> FFEEMTVYAPVPVPVNGNTHYTSESIERLPTGNGNISDLLRTNPAVRMDSTQSTSLNQGDIRPEKISIHGASPYQNAYLIDGISATNNLNPANESDASSATNISGMSQGYYLDVSLLDNVTLYDSFVPVEFGRFNGGVIDAKIKRFNADDSKVKLGYRTTRSDWLTSHIDENNKSAFNQGSSGSTYYSPDFKKNFYTLSFNQELADNFGVTAGLSRRQSDITRADYVSNDGIVAGRAQYKNVIDTALSKFTWFASDRFTHDLTLKYTGSSRDYNTSTFPQSDREMGNKSYGLAWDMDTQLAWAKLRTTVGWDHISDYTRHDHDIWYTELSCTYGDITGRCTRGGLGHISQAVDNYTFKTRLDWQKFAVGNVSHQPYFGAEYIYSDAWTERHNQSESYVINAAGKKTNHTIYHKGKGRLGIDNYTLYMADRISWRNVSLMPGVRYDYDNYLSNHNISPRFMTEWDIFANQTSMITAGYNRYYGGNILDMGLRDIRNSWTESVSGNKTLTRYQDLKTPYNDELAMGLQQKIGKNVIARANYVYREAHDQISKSSRTDSATKTTITEYNNDGKTKTHSFSLSFELAEPLHIRQVDINPQIVFSYIKSKGNLSLNNGYEESNTGDNQVVYNGNLVSYDSVPVADFNNPLKISLNMDFTHQPSGLVWANTLAWQEARKARIILGKTNAQYISEYSDYKQYVDEKLDSSLTWDTRLSWTPQFLQQQNLTISADILNVLDSKTAVDTTNTGVATYASGRTFWLDVSMKF

In Pectobacterium, iron acquisition via plant ferredoxin is mediated by the Ferredoxin uptake system (Fus), a molecular machine consisting of inner and outer membrane transporters and a periplasmically localised protease. Intriguingly, the outer membrane transporter from this system, a TonB-dependent transporter (TBDT) designated FusA, imports intact ferredoxin into the periplasm of the bacteria where it is processed by the M16 family protease FusC. To confirm the common architecture of these systems, we characterised the gene cluster analogous to the Fus from Escherichia coli: the ydd/pqqL operon. Furthermore, through structural and biochemical characterisation of the distantly related Fus homologues, YddB and PqqL from E. coli, we show that these proteins share key features with FusA and FusC, suggesting a conserved function.

In order to determine if FusA homologues possess the structural features required for protein import, we purified and characterised YddB, the FusA homologue from E. coli. YddB belongs to the outer membrane localised TBDT family and has been detected in the outer membrane and in outer membrane vesicles of E. coli in a number of studies. The structure of YddB was solved to a resolution of 2.4 Å by X-ray crystallography by molecular replacement. Based on identification of structural homologues using the Dali server, YddB is most similar to FusA with a RMSD of 2.2 Å and a Z-score of 42.2. As with FusA, YddB possesses a 22-stranded β-barrel fold, the pore of which is occluded by a globular N-terminal plug-domain. This fold is characteristic of the integral outer membrane TBDT family and like these proteins YddB possesses a hydrophobic transmembrane region. Comparison of the structure of YddB and FusA by dissection of their extracellular loops confirmed that the two proteins are structurally analogous; the eleven loops of these proteins share a common structure that is distinct from those of two other TBDTs, FhuE and Fiu. Substrate capture by TBDTs is mediated with an external binding site composed of these extracellular loops. The capture of the large ferredoxin substrate by FusA was shown to be mediated by a large open extracellular binding site. Analysis of the YddB structure revealed that it possesses an analogous binding site, with dimensions (27.8 × 29.2 Å) capable of accommodating a bulky protein substrate of similar dimensions to ferredoxin.> MGSSHHHHHHHHLEVLFQGPHMASLQRKGLQARILTSEEEEKLKRDQTLVSDFKQQKLEQEAQKNWDLFYKRNSTNFFKDRHWTTREFEELRSCREFEDQKLTMLEAGCGVGNCLFPLLEEDPNIFAYACDFSPRAIEYVKQNPLYDTERCKVFQCDLTKDDLLDHVPPESVDVVMLIFVLSAVHPDKMHLVLQNIYKVLKPGKSVLFRDYGLYDHAMLRFKASSKLGENFYVRQDGTRSYFFTDDFLAQLFMDTGYEEVVNEYVFRETVNKKEGLCVPRVFLQSKFLKPPKNPSPVVLGLDPKS

In tRNA, the epigenetic m3C modification at position 32 in the anticodon loop is highly conserved in eukaryotes, which maintains the folding and basepairing functions of the anticodon. A study showed that METTL6 catalyzes the methylation of C32 in several tRNASer isoacceptors. Methylation is most common, and it can be catalyzed by a large family of methyltransferase-like proteins (METTLs) that transfer the methyl group from S-adenosylmethionine (SAM) to a variety of positions in RNA nucleosides. The loss of human METTL6 (hMETTL6) affects the translational process and proteostasis in cells, while in mESCs cells, it leads to defective pluripotency potential.

In this study, we solved the crystal structure of human METTL6 in complex with S-adenosyl-L-homocysteine (SAH) at 1.9 Å and characterized the association mode between the enzyme and the cofactor. The final model ultimately resolved the full-length protein (H-10-P273) except for an internal disordered fragment (T248-C256). The enzyme exhibits a typical Rossmann fold. The helices flanked each side of the central β-sheet formed by seven strands. The SAH ligand fits snuggly in the binding pocket with well-covered density, fixed by the interactions with the enzyme, including hydrogen bonds, salt bridges, and hydrophobic interactions. Specifically, the adenine ring makes multiple hydrogen bonds with the backbone nitrogen of L137, C135, F111, and the terminal carboxyl group of D136, respectively. Additionally, it stacks onto the aromatic ring of F111. The ribose ring also forms three additional hydrogen bonds using its 2′- and 3′- hydroxyl groups, with the side chains of D110 and Y49. Finally, the carboxyl group of SAH accepts a hydrogen bond from H61 while it donates three to G87, I157, and E85, respectively, including some backbone interactions. Lastly, the E85Q mutation reduced the affinity by more than 30-fold, while the D110A mutation almost eliminated the association capacity of the enzyme.Nalpha-{4-[4-(5-chloro-2-methylphenyl)piperazin-1-yl]-2-fluorobenzoyl}-N-pyridin-4-yl-D-tryptophanamide 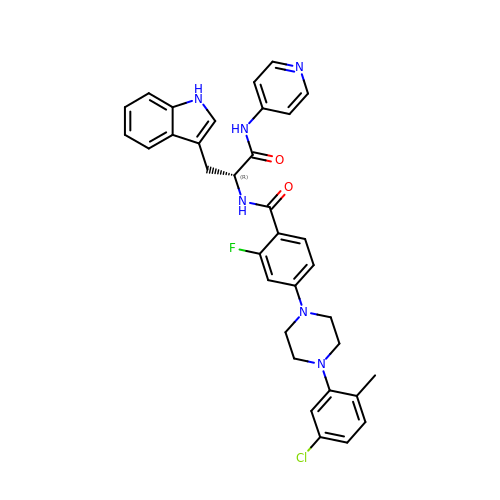| C34 H32 Cl F N6 O2 | JYSKTRNZALHBHU-WJOKGBTCSA-N> MKIAVIGQSLFGQEVYKELKNEGHMIVGVFTIPDKDGKVDPLAIEAEKDGVPVFKFPRWRLKGKAITEVVDQYKAVGAELNVLPFCSQFIPM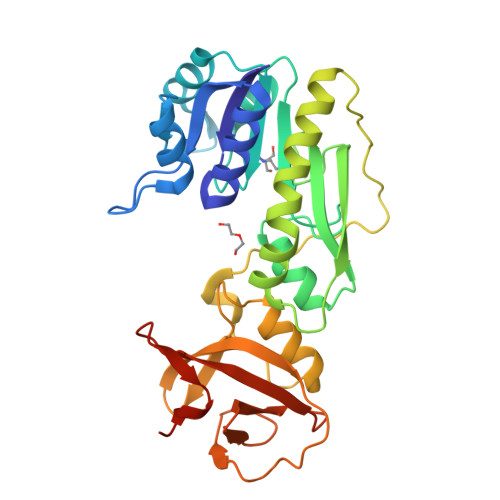EVIDHPKHGSIIYHPSLLPRHRGASAINWTLIHGDKKGGFTVFWADDGLDTGPILLQRECDVEPNDNVNSIYKRFLFPEGVKGMVEAVRLIATGKAPRIKQPEEGATYECIQKKENSKIDWNQPAEAIHNWIRGNDRVPGAWAEIDGKSVSFYGSTLLENDHFSSNGQPLEIPGASRAALVTKNGLVLFGNDGKMLLVKNLQFEDGKMIPGSQYFKAGVEHHHHHH>[2x]GATELHERLAKDSEKLKEEIGKELEELRARLLPHANEVSQKIGDNLRELQQRLEPYADQLRTQVNTQAEQLRRQLT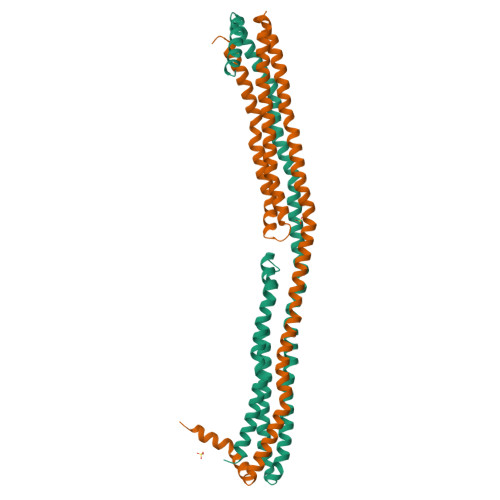PYAQRMERVLRENADSLQASLRPHADELKAKIDQNVEELKGRLTPYADEFKVKIDQTVEELRRSLAPYAQDTQEKLNHQLEGLTFQMKKNAEELKARISASAEELRQRLAPLAEDVRGNLRGNTEGLQKSLAELGGHLDQQVEEFRRRVEPYGENFNKALVQQMEQLRQKLGPHAGDVEGHLSFLEKDLRDKVNSFF>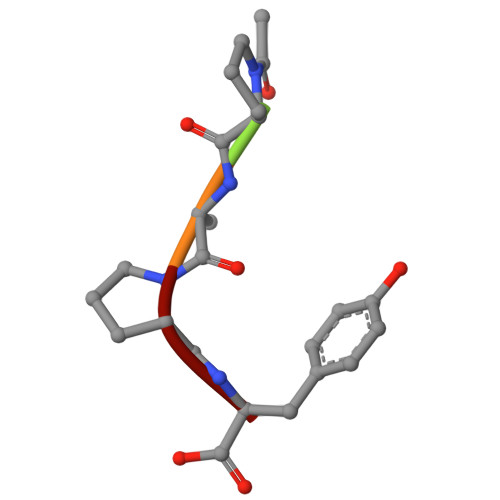 XPAPY> ADKELKFLVVDDFSTMRRIVRNLLKELGFNNVEEAEDGVDALNKLQAGGYGFVISCWNMPNMDGLELLKTIRADGAMSALPVLMVTAEAKKENIIAAAQAGASGYVVKPF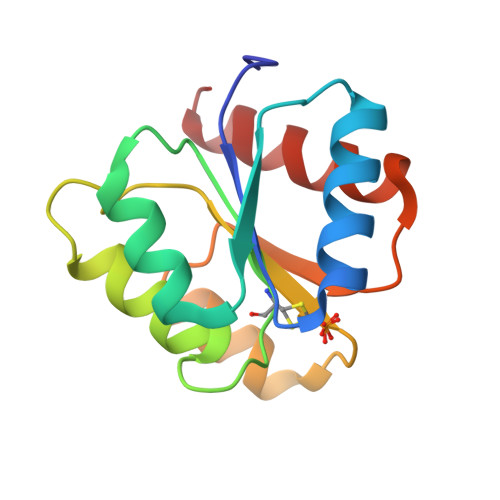TAATLEEKLNKIFEKLGM2-bromo-3-(4-bromophenyl)-4-hydroxy-6-oxo-6,7-dihydrothieno[2,3-b]pyridine-5-carbonitrile 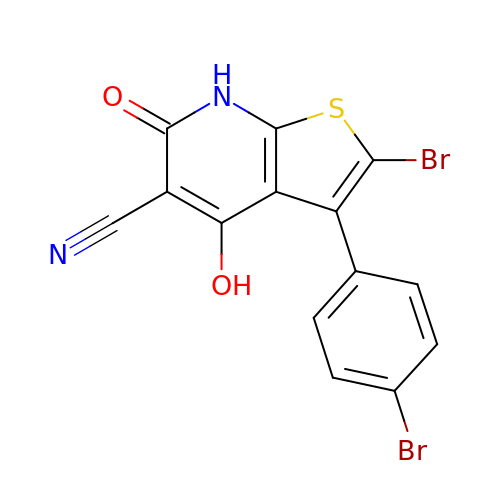| C14 H6 Br2 N2 O2 S | BLJQBTCHXOTSEZ-UHFFFAOYSA-N>[4x]MACLSRIDANLLQYYEKPEPNNTVDLYVSNNSNNNGLKEGDKSISTPVPQPYGSEYSNCLLLSNSEYICYHFSSRSTLLTFYPLSDAYHGKTINIHLPNASMNQRYTLTIQEVEQQLLVNVILKDGSFLTLQLPLSFLFSSANTLNGEWFHLQNPYDFTVRVPHFLFYVSPQFSVVFLEDGGLLGLKKVDGVHYEPLLFNDNSYLKSLTRFFSRSSKSDYDSVISCKLFHERYLIVLTQNCHLKIWDLTSFTLIQDYDMVSQSDSDPSHFRKVEAVGEYLSL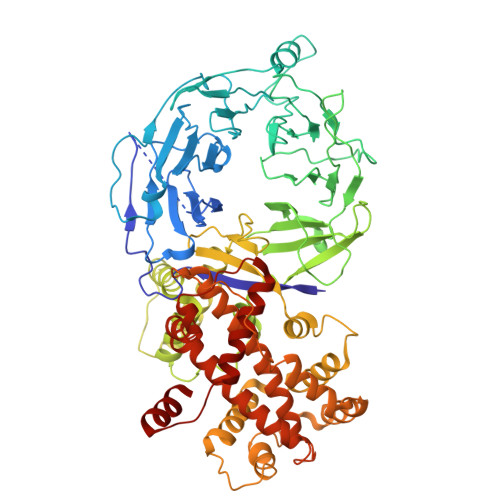YNNTLVTLLPLENGLFQMGTLLVDSSGILTYTFQNNIPTNLSASAIWSIVDLVLTRPLELNVEASYLNLIVLWKSGTASKLQILNVNDESFKNYEWIESVNKSLVDLQSEHDLDIVTKTGDVERGFCNLKSRYGTQIFERAQQILSENKIIMAHNEDEEYLANLETILRDVKTAFNEASSITLYGDEIILVNCFQPYNHSLYKLNTTVENWFYNMHSETDGSELFKYLRTLNGFASTLSNDVLRSISKKFLDIITGELPDSMTTVEKFTDIFKNCLENQFEITNLKILFDELNSFDIPVVLNDLINNQMKPGIFWKKDFISAIKFDGFTSIISLESLHQLLSIHYRITLQVLLTFVLFDLDTEIFGQHISTLLDLHYKQFLLLNLYRQDKCLLAEVLLKDSSEFSFGVKFFNYGQLIAYIDSLNSNVYNASITENSFFMTFFRSYII>MKIGIMSDTHDHLPNIRKAIEIFNDENVETVIHCGDFVSLFVIKEFENLNANIIATYGNNDGERCKLKEWLKDINEENIIDDFISVEIDDLKFFITHGHHQSVLEMAIKSGLYDVVIYGHTHERVFEEVDDVLVINPGECCGYLTGIPTIGILDT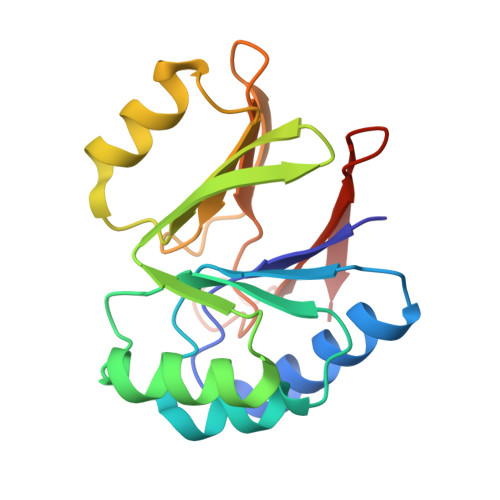EKKEYREIVL[4x]> SPEDFYEVMRLIAVEILNADLEEAHKDQILAEFLNRHFSFSRTNGF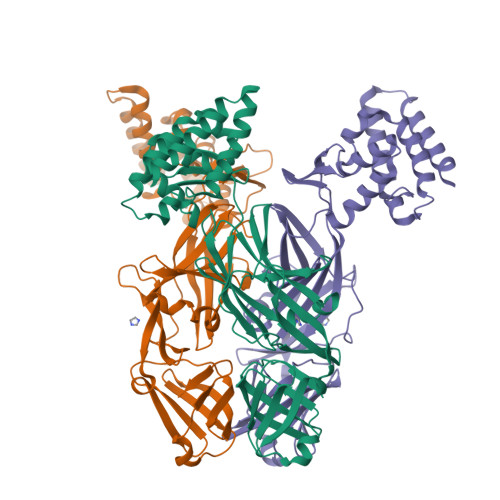SLKVKLEEQPQWINALGDFIQAVPERVDALVMSKLRPLLHYARAKDIDNYRTVEESYRQGQYYRFDIVDGKLNIQFNEGEPYFEGIDIAKPKVKMTAFKFDNHKIVTELTLNEFMIGEGHYDVRLKLHSRNKKHTMYVPLSVNANKQYRFNIMLEDIKAYLPKEKIWDVFLEVQIGTEVFEVRVGNQRNKYAYTAETSALIHLNNDFYRLTPYFTKDFNNISLYFTAITLTDSISMKLKGKNKIILTGLDRGYVFEEGMASVVLKDDMIMGMLSQTSENEVEILLSKDIKKRDFKNIVKLNTAHMTYSLK> MWHYTSINNDTRVALDPKPNQIRTITKPNTVPQLGTDYLYTFNSQRRSHTLRLLGPFQYFNFSETDRGHPLFRLPLKYPSKAIPADELIDNLHSWMRSVHLLHVRSEDNTLRYNWMLGVYARSTNYTTPVGQLVVNAPAILNYSNPQDAFNSVFVALGIDYIDIPITNSNIFDDSSTPYNVRIWHAPTMTEVNHILALMRKSTLVSTHSSWHWNVLHTFHYRSESDMIDHFAAKILEDWRQKEKLDKGALVEADRVIQRLIPLSSSTYVQRLAAIGALYPNEFTENVLDLSRLSTALLQLSDTYYQHANDQLRRLYRRMYNDSRTLYMTQRHQELLLAQITADPNILLYPYTYIFTTIPTSMNYISNTGQGRIKHSLTVTGATEHDTVADIVLGQTGEDVITISMVEPMSIAVEDMYGYVLDTPTRDIWPADEQIEQKGDAVALYDTKTSRALGMFNNTVRIDDLLSPLLSLVYRTYIKGDTMTMTQGSLDHLTLCAAVDSDITFVGNRMIAPLPEGYIPKPMHRNNSTMKMLSLYVALKKLENFATNSYLMAPDTSIILLGAEREPAVNILRRFNRNVSNVRIIGMGDRAVEPNIRVRVPFPIDKNISADFIICDINSYEDQ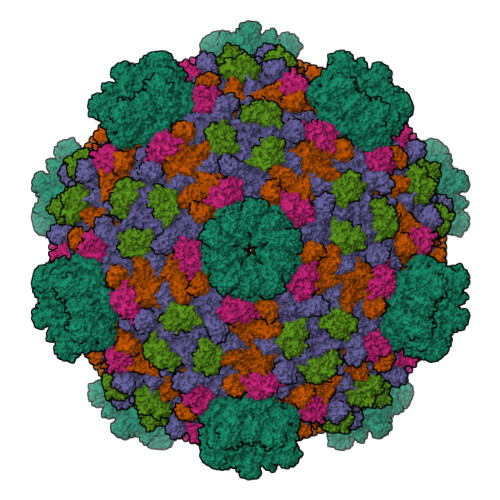SFESMFSETISVVTTCASAATRALVKINHPSEYMINSVIERLSQLGGVFYHTALLKTASQNPYSYETYIYITPIAAAVRFPFYSNSAMINRYMTAVADDEMPIIPSIHTVIKGHSNTYSPGLFCGCVDVQSAPLALSQLKSYCSEATTWRVDSDDNLVNIIARIDPARIALEFRTRSNTSAYHEYQRYVPNGLGFKVRKTREFRYMHREVTFIHKLMMYALIREQISLTENMTQVVSIGGRNLADISVVPLNMKYVVIDPATRIETLTQEKKNIEVQSRPFQFDAANMDLENNSIYLFIAVIMNEPNGAATPARMQMDKIRNVATAMLTRTNCVAYISFYEAGIITRLDQSTAHKTIRVEEGRLKVANYVPVDTLVEADVTLMLRDIGITHEIIRPSTPELIDACSNYGIRLGSTGGAVLDVFNHYSPVIKLVRS;>[2x]MHSTNNNSNKRNNEEKHKQPEIDSSANNGEGTSGTRAQTVGDTATEAGVRNETEAGASTRRQTDGTGLSGTNAKIATASSARQADVEKPADVTFTIENVDDVGIMQQKKPPTVVQSRTDVFNEQFANEALHPTTKVIFNGLDVNTEVQPLSDDFKQISDPKGYLTYSVKYEDQFTKKDKLRASEADDRIVGPTVNLFKYGAAVVNIDLNRDFFDTATGIDLTKGIPLVQDLLVPIGVTAGAEQSAEYVSGLLMVLFKVMTDNRLVIVGETTTPMSNTLSTVVNNVLRTTYHNNVGVNPALLRDFTQVNWLNRDITNMLQQAGTKYGLGLTETRLDYVRLVKTIVGHALNIDHFAASVLNINLRALMEANVTADDRIKALQAHSMISTQFHGPNQGALRPELAFDHDHIIRCLMLAAANYPRLEGIIVQINTGYVASANVIRPVSEKRYFPENLEQNQSAARLVSAVKARASEADISSIHLAIAREVSPMFNVHELKKIAESFEDPSSIVVVLEFILFALFFPTEFNRIKGDIQNVLLLFFSRWYPVEYGIFVQRGATYTINAAGEFEFSGRNEKWDQALYLSEHFPALFSDVPLAGANTIIAIMRLFTPQGFLRTDDLAIAANFPRASRNPQTYIPYTNQRGTVTNEFASRFRTIVATLANVVNERAVQDDMQKATRSCTKQWLRHLETQFDNIAVAHTDHLSVVYATMSNFMLNFTNNFSGNHATFKPDQYVITSPEGSYKPIIERQGETVDGLTIIDTSIVWPILCQCTYPLVRQSGKGVDAVSIMEEIVYPDPSTTLSQSLSVAQVLSKLTLPDAFINMILSGGDSVVMRTYQTEADDDLDEGIRMTTYDQYLSHIRERLHITNVPDPIYITGASTPDQIAASVQATHVAVVLYQSGVINGPASTYLRENEVLVVMPDYYDVVSRFANANLQMNNNRYHESVLEIADIFDQADFIQTSDAVRQLRALMPTLSTSQIRHAIERIAQITDVDSTDYGKLTLRFLGTLTRSLKMQNAQIRRIRPDGTVLRYDDQIDIEAFRWSRYFLDELQLRRLSVGLRLITNPRIARRFNGVRIMYLTDDDPDPDFVPDVPEGYVAVQYAHRLFSSSLANKRNRVTYTHPPTGMAYPSPTGRPHVHMTINERAGMSKLVADNIIASVIKSNWVVDILDIEYTAEVMTPSEGYTQHVDAESIMTAPKGKLFHLQFMDGLLRPEPSAFDPPASGEDMRLIYPLQPISVARSMRAIVNHNEVDRPRGAVAPSSYEMDTGTLSRNGDLLYSPVANGQVGIPKLEVDHISFSNVVSMMTANIRTGDDMAVERVNPDDVRAINIRNA;>MLQQPTGGYTTLEQFAFTIRNDGTNATPTQFLQLLSWEATENELVKKTIPTPETHLPSARNVPGNVYIEDAITQALFGISAQNVNAHGYFSRLSALALPNTSARLGLDGVIYNSETINIPFYDPAAVANFAATYAKLGNASTPRYRADMIDIYAHVGLELAGTDAERAAGVMPVKRAKFDSWEGSLISLSRDVVNWKILAFLIDLCSLEGEALRAFKTRNRDVFRMMLFIMSTAVAANVVNRKVTKRVDRVLEYIGVNSMRTAGRTATITYDLSRHEFAAKFLQLTFTRWNAASAMIRSMPDMHTPRTSITPAGENALVRHNRYMTENFKGLSPIALAQKKHEMMLHTHEIHSMDIDGSIKNMVERETVNKMNEIDAMNTAPWTEEFAEVEPTTVYERHQIGTDPEQTQLISQDAAVIVHQASSDVDENEYGNSVSELTIDTQSDSVL[2x]> GGGARSGDDVVAKYCNACHG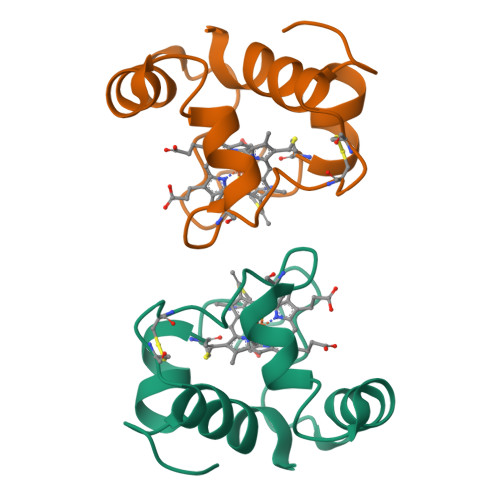TGLLNAPKVGDSAAWKTRADAKGGLDGLLAQSLSGLNAMPPKGTCADCSDDELKAAIGKMSGL> PKFGTHHKALQE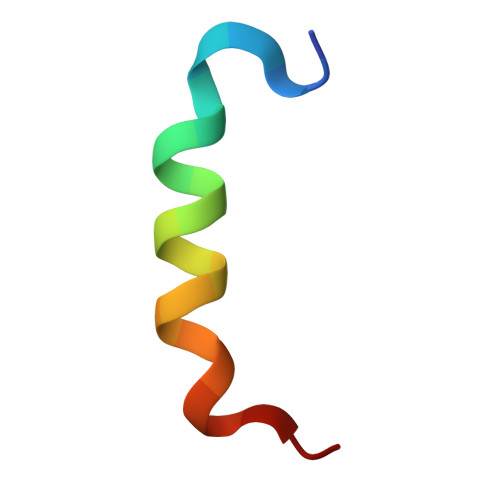IRNSLLPFANE>[2x]GSHMASMEADGRYYSSKQPYVAPNDATASSYSKAPKGYGPIYTESMARHGSRGLSSYKYDALLMRMAETAARDGGFKSEAIKAEFVKNLSGITAANVENGYGMLTGQGAQQHYGIGERAYQRNRSLFDQAAADGGTIAYQSSGEARATESGENFEKGFNEASGGRLIGNVSAPTNPADSGNGKDFQKNPDTLYFHKVQNPDGTSKVPGTKAYDIANNYQNFVANDATIAGAEKTIGDNVDVKRASHDLLSQIFTEEFLAKLENGEYKWYNTTDGTKKGGKNCAPGADASKDPDACGEVSKKIKSEYDAAMDLYNLYIIAADMHNENTGDHTFAFDQYFQGAYADDARMFAWALDAEDFYEKGPSYAGQNETYSIAQPLLDDFLNTIDARVNGGSTVATFRFAHAQT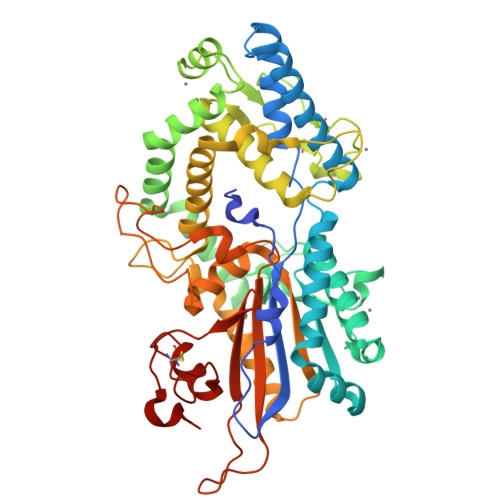MMPFAALLGLPGSTQQAPASTTDVYTYGNNEWRGESVTPMAANVQWDVYARKGEDPATGQRYTPIVRMLYNENEVPFRSECTPVADGSTWYKLTELKSCLAADHKTLGQDARI Tripartite ATP-independent periplasmic (TRAP) transporters are secondary transporters that have evolved an obligate dependence on a substrate-binding protein (SBP) to confer unidirectional transport. We investigated the significance of this interaction using the sialic acid-specific SBP, SiaP, from the Haemophilus influenzae virulence-related SiaPQM TRAP transporter. The first structure of a TRAP SBP revealed that the charge of the carboxylate group of the ligand, sialic acid, was neutralized by an arginine residue, Arg-147, in SiaP, which sequence analysis had revealed to be the most highly conserved residue, being present in 98% of TRAP SBPs of the common DctP family. Using in vitro, in vivo, and structural methods applied to SiaP, we demonstrate that the coordination of the acidic ligand moiety of sialic acid by the conserved arginine (Arg-147) is essential for the function of the transporter as a high affinity scavenging system.

The R147A mutant protein also crystallized in a closed Neu5Ac-bound form, despite effectively reducing the highly conserved charged side chain to a methyl group. In contrast to the R147K mutant, the replacement of Arg-147 by alanine results in removal of all direct contacts between residue 147 and the Neu5Ac. Rather, two water molecules dissipate the charge of the Neu5Ac carboxylate, mediating contacts between ligand and protein. One of these water molecules (water 1) is present in both the R147K and R147A structures, although the other water (water 3) is unique to this structure. Despite this significant change in the binding pocket, the structure of SiaP around the missing arginine is only very mildly perturbed. Water 3 also has a higher B-factor than water 1, which manifests as an anisotropic motion perpendicular to the carboxylate. This mobility translates to the neighboring water molecule (water 4) that moves by ∼1 Å with respect to the wild type, concomitant with a 0.5-Å translation of the β-strand that bears residue 147. There are no additional waters present in the void left by the short side chain of Ala due to the aliphatic patch behind the arginine that drives it into the binding site. Hence, although Arg-147 provides important contacts that are essential for high affinity binding, the required coordination of the Neu5Ac carboxylate in the binding pocket can be fulfilled by water molecules allowing these mutants to both bind and close around the Neu5Ac under these conditions. Interestingly, we observed differential growth phenotypes for the Arg-147 mutants, with the more conservative changes in the R147K mutant exhibiting growth more similar to the strain expressing the wild-type SiaP (doubling times of ∼120 min), than the R147A mutation, which resulted in an ∼50% decrease in the growth rate, giving a doubling time of about ∼180 min.

> ADYDLKFGMNAGTSSNEYKAAEMFAKEVKEKSQGKIEISLYPSSQLGDDRAMLKQLKDGSLDFTFAESARFQLFYPEAAVFALPYVISNYNVAQKALFDTEFGKDLIKKMDKDLGVTLLSQAYNGTRQTTSNRAINSIADMKGLKLAVPNAATNLAYAKYVGASPTPMAFSEVYLALQTNAVDGQENPLAAVQAQKFYEVQKFLAMTNHILNDQLYLVSNETYKELPEDLQKVVKDAAENAAKYHTKLFVDGEKDLVTFFEKQGVKITHPDLVPFKESMKPYYAEFVKQTGQKGESALKQIEAINPHHHHHH>[2x]SMTRTYDREGFKKRAACLCFRSEQEDEVLLVSSSRYPDQWIVPGGGMEPEEEPGGAAVREVYEEAGVKGKLGRLLGIFENQDRKHRTYVYVLTVTEILED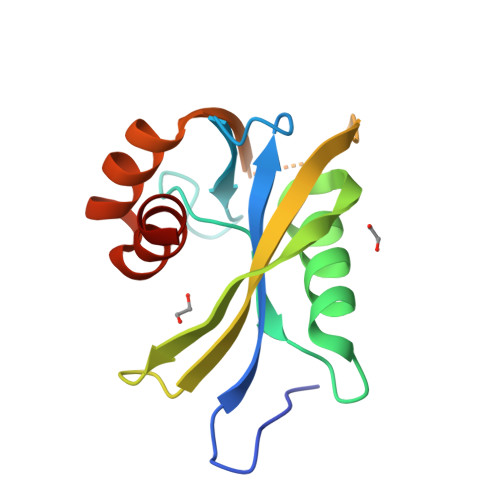WEDSVNIGRKREWFKVEDAIKVLQCHKPVHAEYLEKLKLG In pseudocyclic proteins, such as TIM barrels, β barrels, and some helical transmembrane channels, a single subunit is repeated in a cyclic pattern, giving rise to a central cavity that can serve as a pocket for ligand binding or enzymatic activity. Inspired by these proteins, we devised a deep-learning-based approach to broadly exploring the space of closed repeat proteins starting from only a specification of the repeat number and length. Biophysical data for 38 structurally diverse pseudocyclic designs produced in Escherichia coli are consistent with the design models, and the three crystal structures we were able to obtain are very close to the designed structures. The large set of pseudocycles with central binding pockets described here combines the diversity of native protein scaffolds with the stability and robustness of de novo-designed proteins, and our RIF docking and Rosetta design calculations suggest that the designed pseudocycles provide better starting scaffolds for small-molecule binder design than do either native structures or previously designed de novo NTF2s.

a–e, Crystal structures of the five-repeat design E8 (a), two-repeat design H12 (b), and the three-repeat design H10 (c–e) are shown as gray cartoons; the loop, sheets, and helix of the design are shown in dark blue, magenta, and teal, respectively. Central pockets in the designs are shown as gray spheres (a–c). The approach generates a wide variety of structures strongly encoded by their amino acid sequences (as evaluated with RF and AF2, and further indicated by the close agreement between the crystal structures and design models), with between 2 and 7 repeat units (N), repeat lengths of 15 to 78 (L), and all ɑ-, ɑ/β-, and all β-folds.

>SGSPTPLETLPLEELERRALKIYLRRHGSVPEEEIETMPLEELERKALQDYLRRYGTLPEEEIETMPLEELEREALKNYLRRYGTLPEEEIDTMPLEELEREALKNYLRRYGSLPPEELEKLPLEELERKALIEYLRRYGPSGSG[2x]> GSPEFMIGEEVPSDQYYWAPLAQHERGSLASLDSLRKGGPPPPNWRQPELPEVIAMLGFRLDAVKSNAAAYLQHLCYRNDKVKTDVRKLKGIPVLVGLLDHPKKEVHLGACGALKNISFGRDQDNKIAIKNCDGVPALVRLLRKARDMDLTEVITGTLWNLSSHDSIKMEIVDHALHALTDEVIIPHSGWEREPNEDCKPRHIEWESVLTNTAGCLRNVSSERSEARRKLRECDGLVDALIFIVQAEIGQKDSDSKLVENCVCLLRNLSYQVHREIPQAERYQEAAPNVANNTGTSPARGYELLFQPEVVRIYISLLKESKTPAILEASAGAIQNLCAGRWTYGRYIRSALRQEKALSAIADLLTNEHERVVKAASGALRNLAVDARNKELIGKHAIPNLVKNLPGGQQNSSWNFSEDTVISILNTINEVIAENLEAAKKLRETQGIEKLVLINKSGNRSEKEVRAAALVLQTIWGYKELRKPLEKEGWKKSDFQVNLNNASRSQSSHSYDDSTLPLIDRNQKSDKKPDREEIQMS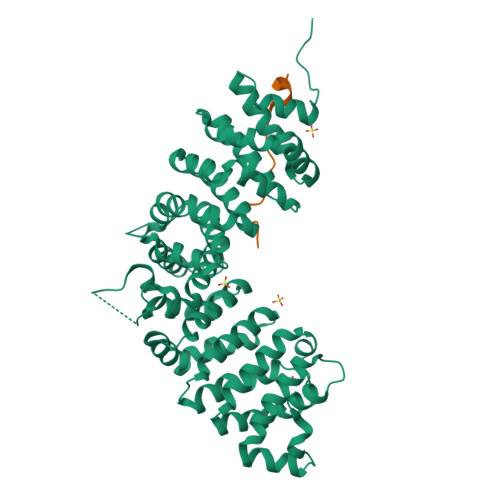NMGSNTKSLDNNYSTPNERGDHNRTLDRSGDLGDMEPLKGTTPLMQKI;> DEEGGGEEDQDFDLSQLH>[2x]KHTLPDLPFDYADLEPVISHEIMQLHHQKFHATYVNNLNQIEEKLHEAVSKGNLKEAIALQPALKFNGGGHINHSIFWTNLAKDGGEPSKELMDTIKRDFGSLDNLQKRLSDITIAV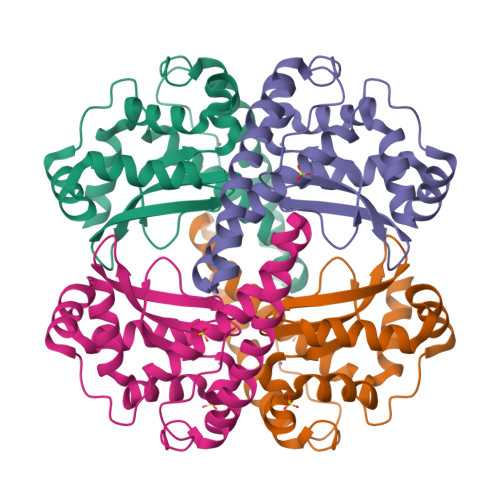QGSGWGWLGYCKKDKILKIATCANQDPLEGMVPLFGIDVWEHAYYLQYKNVRPDYVHAIWKIANWKNISERFANARQ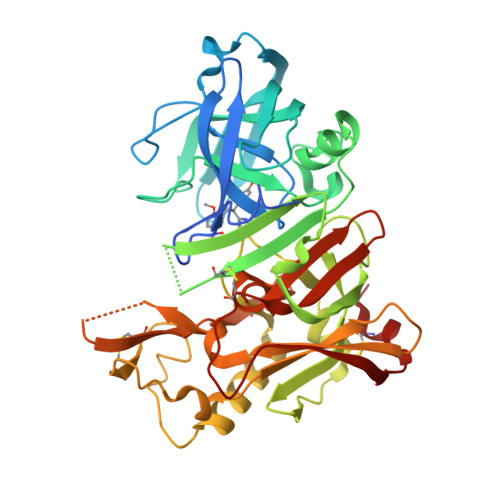>[3x]MLPRETDEEPEEPGRRGSFVEMVDNLRGKSGQGYYVEMTVGSPPQTLNILVDTGSSNFAVGAAPHPFLHRYYQRQLSSTYRDLRKGVYVPYTQGKWEGELGTDLVSIPHGPNVTVRANIAAITESDKFFINGSNWEGILGLAYAEIARPDDSLEPFFDSLVKQTHVPNLFSLQLCGAGFPLNQSEVLASVGGSMIIGGIDHSLYTGSLWYTPIRREWYYEVIIVRVEINGQDLKMDCKEYNYDKSIVDSGTTNLRLPKKVFEAAVKSIKAASSTEKFPDGFWLGEQLVCWQAGTTPWNIFPVISLYLMGEVTNQSFRITILPQQYLRPVEDVATSQDDCYKFAISQSSTGTVMGAVIMEGFYVVFDRARKRIGFAVSACHVHDEFRTAAVEGPFVTLDMEDCGYN> MHHHHHHLVPRGSMLDFEKPLFEIRNKIESLKESQDKNDVDLQEEIDMLEASLERETKKIYTNLKPWDRVQIARLQERPTTLDYIPYIFDSFMELHGDRNFRDDPAMIGGIGFLNGRAVTVIGQQRGKDTKDNIYRNFGMAHPEGYRKALRLMKQAEKFNRPIFTFIDTKGAYPGKAAEERGQSESIATNLIEMASLK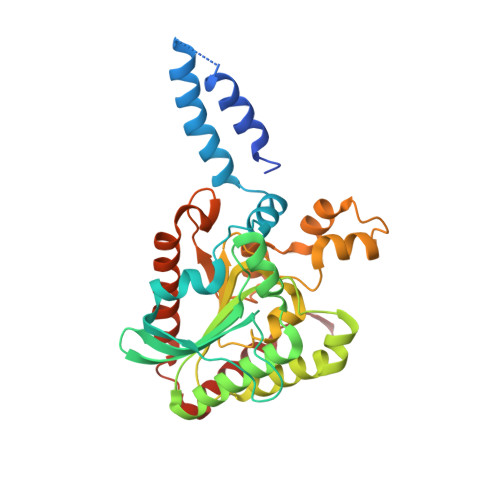VPVIAIVIGEGGSGGALGIGIANKVLMLENSTYSVISPEGAAALLWKDSNLAKIAAETMKITAHDIKQLGIIDDVISEPLGGAHKDIEQQALAIKSAFVAQLDSLESLSRDEIANDRFEKFRNIGSYIE>[2x]MSLDGMPAKQQHNNTGESVELHFHYPIKGKQEPKNSHLVVLIEPKIEINKVIPESYQKEFEKSLFLQLSSFLERKGYSVSQFKDASEIPQD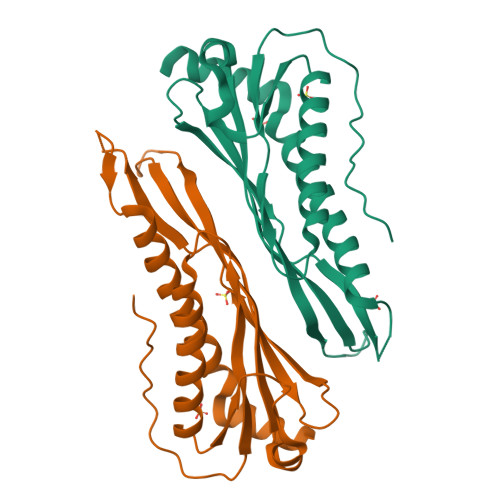IKEKALLVLRMDGNVAILEDIVEESDALSEEKVIDMSSGYLNLNFVEPKSEDIIHSFGIDVSKIKAVIERVELRRTNSGGFVPKTFVHRIKETDHDQAIRKIMNQAYHKVMVHITKELSKKHMEHYEKVSSEMKKRKEGHHHHHH> MSENKAPGQIYAYDIHNTHYPYVNIKQDSQTQLLASFRRSIASINPFSYRQVPSQDRAAFGLRWGNAWYAPNPYPNGIHFDRVFPTHYDPLAETNRTKANLQLIKYAPGNYSTLVVTSEKLPRPCIRTIQNYRRCQMVNGTEKCNSEAQDILAICPNWALDHMKEKVRFYTKALAINNQTYIRAMQVEEYNQGRTVADVAPKTWIHGTRQHLRPDTMWADDRYTNITQTEINEAIKRVEARKAREHEKKPVEQANVNANTGEQ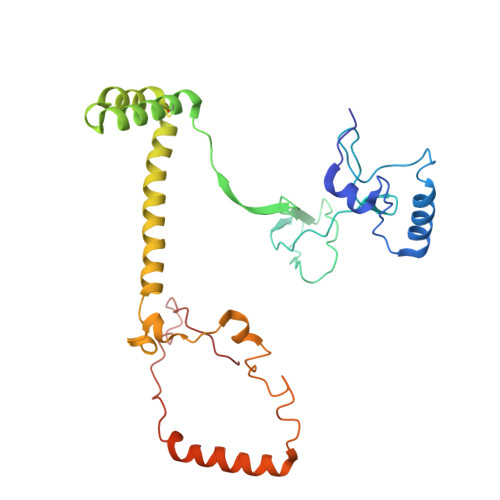PVRVEKSLYP>MDIGINSDMTGKRQFPDDFIWGAATASYQIEGAANEGGRGPSIWDTFSKTPGKVLLGHTGDVACDHFHRYESDVKLMADLGIKSYRFSLAWPRVMPEKGRYLESGFDFYKRLIEQLHKHGITPAATIYHWDLPQWIEDEGGWSNRAVVDYYKEFAEQAFKALGDDVPFWITHNEPWCASLLSYGIGEHAPGLKDWRRAYRAAHHILLSHGEAVKLYRELGLKGQIGITLNLTPAYPASDSPEDIAAQQRQDAFSNRWFLDPIFKGEYPADFMPRVERFCGDLNVIQPGDMETISVPQDFLGINFYTRSVVKDDPADDSLISVHGVPTDNPVTDMGWE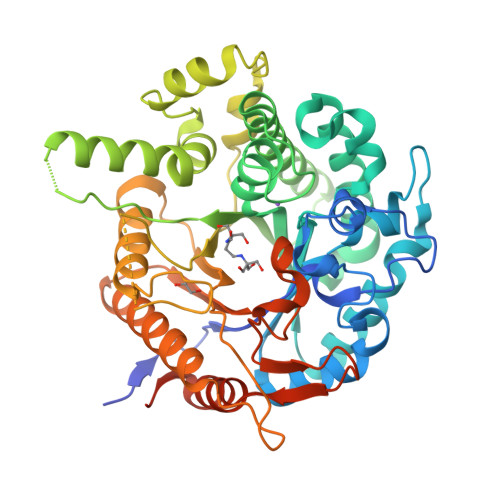IYPDALYDLLHRLKNEYTDLPIYITENGAANADAIVNGEVEDTPRIDYVRQHLDAAHRFIQEGGNLKGYYLWSLMDNFEWAFGYTKRFGIIYVDYETQVRTPKASFHWYRQVIENNGLTDKLAAAENLYFQGLEHHHHHH[8x]>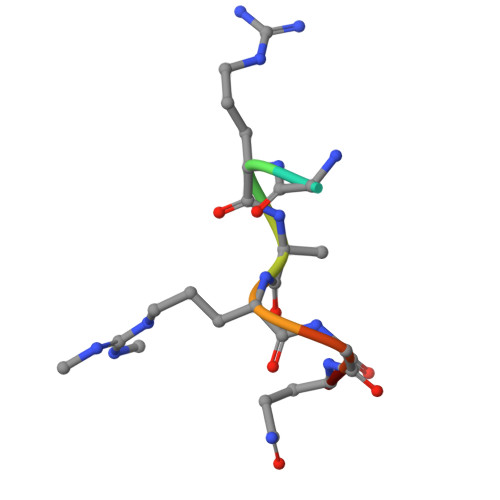 RGRARGQE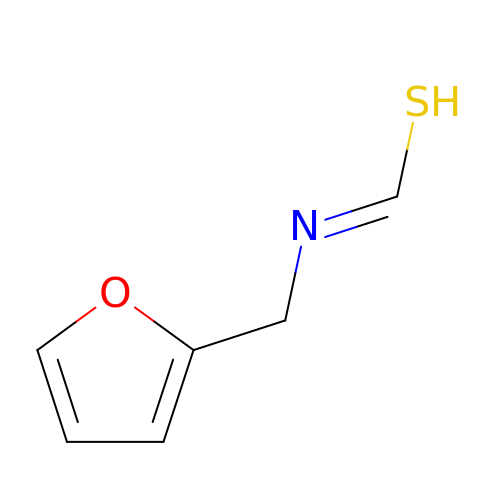(Z)-[(furan-2-ylmethyl)imino]methanethiol | C6 H7 N O S | BDAKRWHGDWIWEU-UHFFFAOYSA-N>[2x]MWKRSEQMKIKSGKCNMAAAMETEQLGVEIFETADCEENIESQDRPKLEPFYVERYSWSQLKKLLADTRKYHGYMMAKAPHDFMFVKRNDPDGPHSDRIYYLAMSGENRENTLFYSEIPKTINRAAVLMLSWKPLLDLFQATLDYGMYSREEELLRERKRIGTVGIASYDYHQGSGTFLFQAGSGIYHVKDGGPQGFTQQPLRPNLVETSCPNIRMDPKLCPADPDWIAFIHSNDIWISNIVTREERRLTYVHNELANMEEDARSAGVATF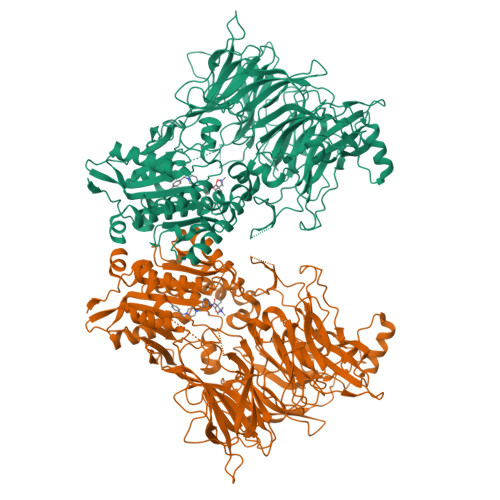VLQEEFDRYSGYWWCPKAETTPSGGKILRILYEENDESEVEIIHVTSPMLETRRADSFRYPKTGTANPKVTFKMSEIMIDAEGRIIDVIDKELIQPFEILFEGVEYIARAGWTPEGKYAWSILLDRSQTRLQIVLISPELFIPVEDDVMERQRLIESVPDSVTPLIIYEETTDIWINIHDIFHVFPQSHEEEIEFIFASECKTGFRHLYKITSILKESKYKRSSGGLPAPSDFKCPIKEEIAITSGEWEVLGRHGSNIQVDEVRRLVYFEGTKDSPLEHHLYVVSYVNPGEVTRLTDRGYSHSCCISQHCDFFISKYSNQKNPHCVSLYKLSSPEDDPTCKTKEFWATILDSAGPLPDYTPPEIFSFESTTGFTLYGMLYKPHDLQPGKKYPTVLFIYGGPQVQLVNNRFKGVKYFRLNTLASLGYVVVVIDNRGSCHRGLKFEGAFKYKMGQIEIDDQVEGLQYLASRYDFIDLDRVGIHGWSYGGYLSLMALMQRSDIFRVAIAGAPVTLWIFYDTGYTERYMGHPDQNEQGYYLGSVAMQAEKFPSEPNRLLLLHGFLDENVHFAHTSILLSFLVRAGKPYDLQIYPQERHSIRVPESGEHYELHLLHYLQENLGSRIAALKVI>[6x]MSLSASLGATRFRPDLLSLDDLDEAQLHALLTLAHQLKRGERVANLHGKVLGLVFLKASTRTRVSFTVAMYQLGGQVID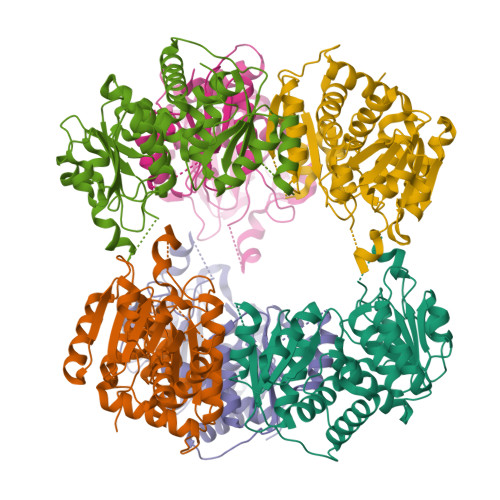LSPSNTQVGRGEPVRDTARVLGRYVDGLAIRTFAQTELEEYAHYAGIPVINALTDHEHPCQVVADLLTIRENFGRLAGLKLAYVGDGNNVAHSLLLGCAKVGMSIAVATPEGFTPDPAVSARASEIAGRTGAEVQILRDPFEAARGAHILYTDVWTSMGQEAETQHRLQLFEQYQINAALLNCAAAEAIVLHCLPAHRGEEITDEVMEGPRSRIWDEAENRLHAQKAVLAALMGGREGHHHHHH>GHMNDLIDTTEMYLRTIYDLEEEGVVPLRARIAERLEQSGGTVSQTVARMERDGLLTVAEDRHLELTKAGRARAISVMRKHRLAERLLVDVIGLEWEQVHLEACRWEHVMSEAVERKLVKLLGNPTTSPYGNPIPGLDELGVGDSVEPVDTDLRRVDEVARSGGGRALVCRIAEHVQLDPDLMSELKKVGVVPGNEIDIVAVAGVNKPIQVQGSEGGTQLQPGIAHAVMVRVK[6x]

The iron-dependent regulator IdeR is the main transcriptional regulator controlling iron homeostasis genes in Actinobacteria, including species from the Corynebacterium, Mycobacterium and Streptomyces genera, as well as the erythromycin-producing bacterium Saccharopolyspora erythraea. IdeR is an OCS from the DtxR (Diphtheria toxin repressor) family of transcriptional regulators which typically consist of three domains: an N-terminal DNA-binding winged helix-turn-helix (wHTH) motif, followed by a dimerization interface that contains most of the metal-binding residues, and a C-terminal SH3-like domain (21–23). The main function of IdeR is to repress the expression of iron uptake genes when the intracellular iron levels are sufficient. When iron levels are sufficient for iron ions to occupy the IdeR metal-binding sites, the regulator is activated and recognizes a highly conserved 19-bp sequence located in the promoter region of its target genes.

To clarify the relevance of the base interactions with the recognition helix of IdeR, we generated two IdeR variants, IdeRQ43A and IdeRP39G, that should disrupt base interactions while not affecting backbone interactions. As for the IdeRP39G variant, the EMSA results show specific binding to the consensus target, but the affinity is significantly affected by the mutation, resulting in an apparent KD of ∼264 nM. Due to the special structural features of both proline and glycine residues we cannot conclude whether this loss of affinity is caused by the absence of the vdW interactions with the DNA, or if this protein variant is functionally impaired. However, as IdeRP39G is still able to recognize its target and form a stable complex, we can reason that the absence of IdeRWT binding to the Consensus_T3-G3 sequence was not caused by the disruption of the vdW interactions between Pro39 and the thymine in position 3. We also obtained the crystal structure of IdeRP39G bound to the consensus DNA to confirm that no other interactions with the essential thymines of the recognition sequence are formed in this IdeR variant. Despite the drastic difference between the wild-type and mutated residue, in the DNA-bound state the structure of the recognition helix is essentially unaffected by the mutation. The hydrogen bond formed by the backbone carbonyl group of residue 39 with the water molecule, which is also bound to Gln43 and the cytosine in position 2 of the repeat, is not disrupted by the mutation.> MIPGEYH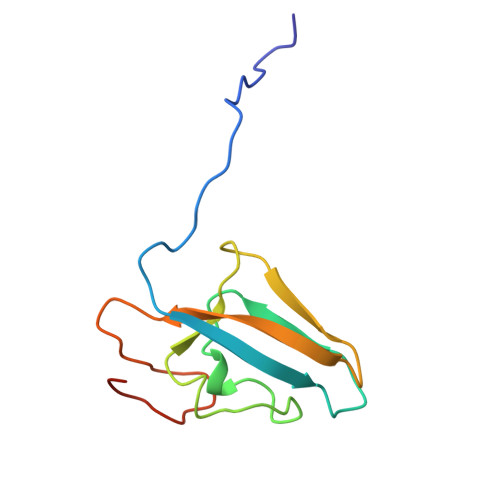VKPGQIALNTGRATCRVVVENHGDRPIQVGSHYHFAEVNPALKFDRQQAAGYRLNIPAGTAVRFEPGQKREVELVAFAGHRAVFGFRGEVMGPLEVNDE The plant-type carotene desaturation system is mechanistically linked to redox chains in which quinones, the alternative oxidase PTOX and molecular oxygen participate. This is contrasted by the phytoene desaturases of the CRTI-type prevailing in archaea, bacteria and fungi which are capable of catalyzing the entire desaturation sequence including one cis-to-trans isomerization reaction at the central double bond (Figure 1; for review, see [16]). For the conversion of colorless 15-cis-phytoene into red-colored all-trans-lycopene CRTI thus takes over the function of at least four enzymes employed by cyanobacteria and plants. The observation that highly purified phytoene desaturase CRTI-His6 from Pantoea ananatis very efficiently converts 15-cis-phytoene into all-trans-lycopene in the presence of FAD and in the absence of any other cofactors or metals speaks for FAD being the sole redox catalyst involved. Since in CRTI-mediated desaturation in vitro redox equivalents are transferred from phytoene via FAD to oxygen the system behaves formally as an oxidase.

Native, enzymatically active CRTI was crystallized in the space group P3221 with one monomer in the asymmetric unit. The structure of apo-CRTI was solved at 3.0 Å by multiple anomalous dispersion using selenomethionine derivatives. The model was further refined against a 2.35 Å resolution native data set to an R-factor of 19.1% and an R-free of 22.9%. The structure of apo-CRTI is composed of 19 β-strands (forming 5 sheets), 12 alpha-helices, and three 310-helices. Altogether these fold into three pseudo-domains consistent with the flavin containing amino oxidoreductase family (Pfam: PF01593) as revealed by structural search comparisons (see the topology diagram and structural alignment in Figure S3 and Figure 10, respectively). The first, the FAD binding domain is composed of a five-stranded, parallel sheet sandwiched between a three-stranded anti-parallel sheet and a five-helix bundle. The ligand binding domain is composed of a seven-stranded mixed topology sheet with two alpha-helices packed onto the top surface and two, two-stranded anti-parallel sheets and two 310-helices packed onto one edge of the bottom surface of the sheet. The third domain packs against the rest of the bottom surface of sheet 4 and is composed of a six-helix bundle. The final model showed several disordered regions, and of the 492 CRTI residues only 404 are visible in the electron density map. No density could be seen for residues 34–40, 138–139, 195–196, 275–302, 331–343, 426–455, 465–470. Structural analyses revealed that most of the disordered regions (i.e. 34–40, 275–302, 426–455, 465–470) are involved in the predicted FAD binding site and therefore order-to-disorder transition should occur upon FAD binding and membrane binding (see above).

> MKPTTVIGAGFGGLALAIRLQAAGIPVLLLEQRDKPGGRAYVYEDQGFTFDAGPTVITDPSAIEELFALAGKQLKEYVELLPVTPFYRLCWESGKVFNYDNDQTRLEAQIQQFNPRDVEGYRQFLDYSRAVFKEGYLKLGTVPFLSFRDMLRAAPQLAKLQAWRSVYSKVASYIEDEHLRQAFSFHSLLVGGNPFATSSIYTLIHALEREWGVWFPRGGTGALVQGMIKLFQDLGGEVVLNARVSHMETTGNKIEAVHLEDGRRFLTQAVASNADVVHTYRDLLSQHPAAVKQSNKLQTKRMSNSLFVLYFGLNHHHDQLAHHTVCFGPRYRELIDEIFNHDGLAEDFSLYLHAPCVTDSSLAPEGCGSYYVLAPVPHLGTANLDWTVEGPKLRDRIFAYLEQHYMPGLRSQLVTHRMFTPFDFRDQLNAYHGSAFSVEPVLTQSAWFRPHNRDKTITNLYLVGAGTHPGAGIPGVIGSAKATAGLMLEDLIGGSHHHHHH>MTTSASSHLNKGIKQVYMSLPQGEKVQAMYIWIDGTGEGLRCKTRTLDSEPKCVEELPEWNFDGSSTLQSEGSNSDMYLVPAAMFRDPFRKDPNKLVLCEVFKYNRRPAETNLRHTCKRIMDMVSNQHPWFGMEQEYTLMGTDGHPFGWPSNGFPGPQGPYYCGVGADRAYGRDIVEAHYRACLYAGVKIAGTNAEVMPAQWEFQIGPCEGISMGDHLWVARFILHRVCEDFGVIATFDPKPIPGNWNGAGCHTNFSTKAMREENGLKYIEEAIEKLSKRHQYHIRAYDPKGGLDNAARLTGFHETSNINDFSAGVANRSASIRIPRTVGQEKKGYFEDRRPSANCDPFSVTEALIRTCLLNETGDEPFQYKN[10x]

Glutamine synthetase (GS) is an ancient enzyme that catalyzes the ATP-dependent condensation of glutamate and ammonia to glutamine (Eisenberg et al. 2000; de Carvalho Fernandes, Turchetto-Zolet, and Pereira Passaglia 2022; Tecson et al. 2025). Here, we demonstrate that human glutamine synthetase (GS) can reversibly polymerize into filaments aided by a composite binding site formed at the filament interface by the product, glutamine. The glutamate/ammonia binding site is gated by a flexible loop that bears two key catalytic residues: R299, which interacts with glutamate substrate carboxyl group, and E305, which is predicted to deprotonate ammonium ions to ammonia, enabling the required nucleophilic attack of the y-glutamyl phosphate intermediate. We propose that GS filament formation constitutes a negative-feedback mechanism, directly linking product concentration to the structural and functional remodeling of the enzyme.

To test the model that loop biasing impacts KM values for GS, we structurally characterized the decameric form of loop variant R298A under turnover conditions. The final reconstruction yielded an overall map of FSC0.143 of 1.95 Å with high local resolution values across the map. Importantly, this map, despite being the highest global resolution map reconstructed, did not display any appreciable E305-loop density, similar to the turnover filament. Thus, the R298A mutant, even in the decameric form, would rarely adopt the active-closed conformation, explaining the KM, glutamate and KM, ammonia defects resulting from this mutation. We observe multiple residue contacts that appear stabilizing including a hydrophobic pocket formed by L300, I285, and I309, a salt-bridge formed between R298 and D239, and a hydrogen bond between H304 and N249. Disruption of the hydrophobic interface of L300, I309, and I285 appeared to have largest impact on KM, glutamate, followed by disruption of the R298*D239 salt bridge (50-fold change for both variants), followed lastly by disruption of the H304*N249 hydrogen bond. However, the two loop mutants, R298A and L300A, could not support growth under glutamine-deplete conditions displaying the same phenotype as P242stop. The KM, glutamate for R298A and L300A are outside the normal steady state concentrations of intracellular glutamate, suggesting that loop conformational control of the Michaelis-complex can occur in the cell to directly impact metabolic flux through GS.> HPYYLRSFLVVLKTVLENEDDMLLFDEQEKGIVTKFYQLSATGQKLYVRLFQRKLSWIKMTKLEYEEIALDLTPVIEELTNAGF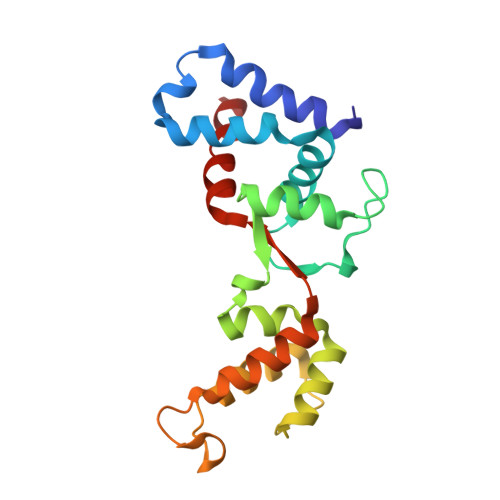LQTESELQELSEVLELLSAPELKSLAKTFHLVNPNGQKQQLVDAFLKLAKQRSVCTWGKNKPGIGAVILKRAKALAGQSVRICKGPRAVFSRILLLFSL> GHMAMEFSSVGTHRFVQKVEEMVQNHMTYSLQDVGGDANWQLVVEEGEMKVYRREVEENGIVLDPLKATHAVKGVTGHEVCNYFWNVDVRNDWETTIENFHVVETLADNAII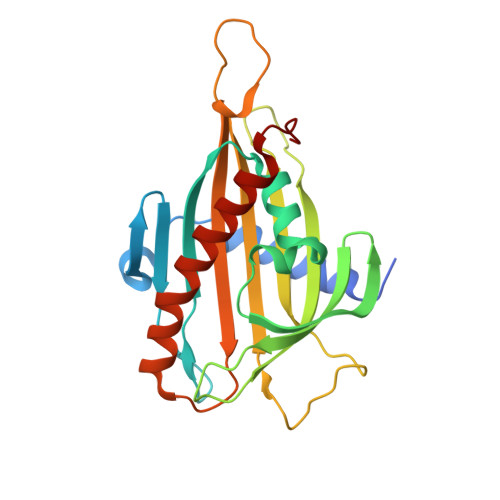IYQTHKRVWPASQRDVLYLSVIRKIPALTENDPETWIVCNFSVDHDSAPLNNRCVRAKINVAMICQTLVSPPEGNQEISRDNILCKITYVANVNPGGWAPASVLRAVAKREYPKFLKRFTSYVQEKTAGKPILF>[2x]QVTVIPR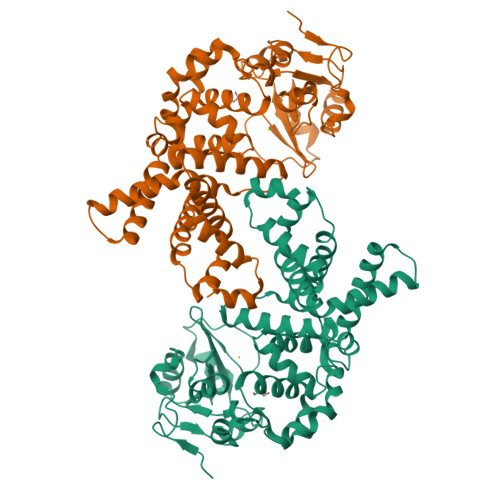EQHAISRKDISENALKVMYRLNKAGYEAWLVGGGVRDLLLGKKPKDFDVTTNATPEQVRKLFRNCRLVGRRFRLAHVMFGPEIIEVATFRGHHEGNVSDRTTSQRGQNGMLLRDNIFGSIEEDAQRRDFTINSLYYSVADFTVRDYVGGMKDLKDGVIRLIGNPETRYREDPVRMLRAVRFAAKLGMRISPETAEPIPRLATLLNDIPPAHLFEESLKLLQAGYGYETYKLLCEYHLFQPLFPTITRYFTENGDSPMERIIEQVLKNTDTRIHNDMRVNPAFLFAAMFWYPLLETAQKIAQESGLTYHDAFALAMNDVLDEACRSLAIPKRLTTLTRDIWQLQLRMSRRQGKRAWKLLEHPKFRAAYDLLALRAEVERNAELQRLVKWWGEFQVSAPPDQKGMLNELD>[4x]GPGLKQKIVIKVAMEGNNCRSKAMALVASTGGVDSVALVGDLRDKIEVVGYGIDPIKLISALRKKVGDAELLQVSQAKED;>ETGNKYIEKRAIDLSRERDPNFFDNPGIPVPECFWF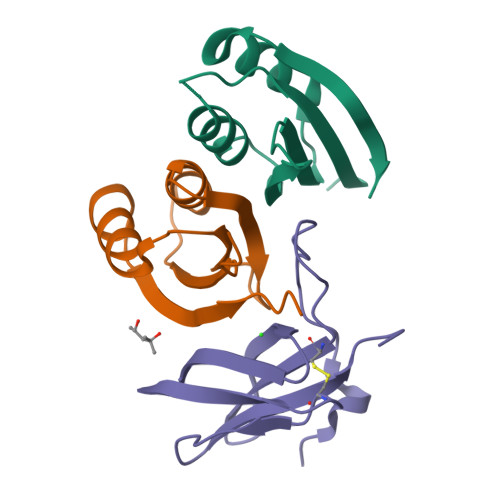MFKNNVRQDAGTCYSSWKMDMKVGPNWVHIKSDDNCNLSGDFPPGWIVLGKKRPGF[2x]> TFTAKTGTNFGNDNDAEAYLQFEKLIDKKYLKLPTRVNLEILRGTKIHSSFLFNSYSSLSPQSILNLKVFSQFYNWNTNKGLDIGQRGARLSLRYEPLFLHKLLHNPHSNESPTLFHEWFLETCWRSTKICSQGTSAPYMYSGTMLSQAGDQLRTILGHTFVLDKRDHIMCPTKGSMLKWSNELSPGKHLKTQLELNSVKSWMNDDFITFSTTIKTGYLKNLSSQQSLPVHICDKFQSGGPSDIRGFQTFGLGPRDLYDAVGGDAFVSYGLSVFSRLPWKKVEKSNFRLHWFFNGGKLVNHDNTSLGNCIGQLSKEHSTSTGIGLVLRHPMARFELNFTLPITAHENDLIRKGFQFGLGLAFL;> MVSSFSVPMPVKRIFDTFPLQTYAAQTDKDEAVALEIQRRSYTFTERGGGSSELTVEGTYKLGVYNVFLEANTGAALATDPWCLFVQLALCQKNGLVLPTHSQEQTPSHTCNHEMLVLSRLSNPDEALPILVEGYKKRIIRSTVAISEIMRSRILDDAEQLMYYTLLDTVLYDCWITQIIFCASDAQFMELYSCQKLSGSIVTPLDVENSLLQKLSAKSLKISLTKRNKFQFRHREIVKSMQGVYHNHHNSVNQEQVLNVLFENSKQVLLGLKDMLKSDGQPTYLHLKIASYILCITNVKEPIKLKTFVENECKELVQFAQDTLKNFVQ;> MVKG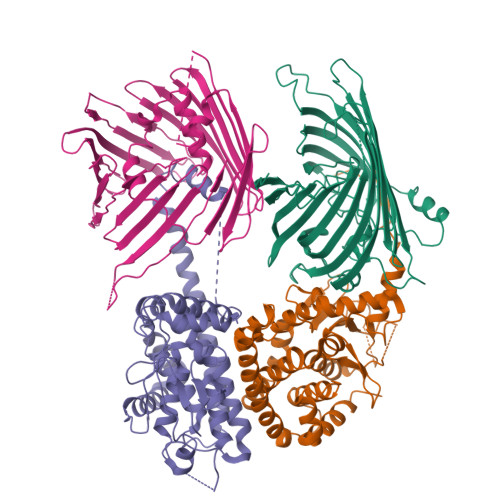SVHLWGKDGKASLISVDSIALVWFIKLCTSEEAKSMVAGLQIVFSNNTDLSSDGKLPVLILDNGTKVSGYVNIVQFLHKNICTSKYEKGTDYEEDLAIVRKKDRLLEYSLLNYVDVEISRLTDYQLFLNTKNYNEYTKKLFSKLLYFPMWYNTPLQLRSQARENCEEIIGSLTLEDDEEFVESKAMESASQLAQSKTFKIAHKNKIKGKQELQQVKYNLQFDNRLQSCVSNWLAARKKLDDSVILSSDLLFLANLYVQLGLPDGNRIRSKLEQTFGSELLNSMSNKIDDFVHRPSNNLEQRDPQFREQGNVVMSLYNLACKYI;> MLPYMDQVLRAFYQSTHWSTQNSYEDITATSRTLLDFRIPSAIHLQISNKSTPNTFNSLDFSTRSRINGSLSYLYSDAQQLEKFMRNSTDIPLQDATETYRQLQPNLNFSVSSANTLSSDNTTVDNDKKLLHDSKFVKKSLYYGRMYYPSSDLEAMIIKRLSPQTQFMLKGVSSFKESLNVLTCYFQRDSHRNLQEWIFSTSDLLCGYRVLHNFLTTPSKFNTSLYNNSSLSLGAEFWLGLVSLSPGCSTTLRYYTHSTNTGRPLTLTLSWNPLFGHISSTYSAKTGTNSTFCAKYDFNLYSIESNLSFGCEFWQKKHHLLETNKNNNDKLEPISDELVDINPNSRATKLLHENVPDLNSAVNDIPSTLDIPVHKQKLLNDLTYAFSSSLRKIDEERSTIEKFDNKINSSIFTSVWKLSTSLRDKTLKLLWEGKWRGFLISAGTELVFTRGFQESLSDDEKNDNAISISATDTENGNIPVFPAKFGIQFQYST>[2x]MRQIAIYGKGGIGKSTTTQNLTAALSTMGNNILLVGCDPKADSTRMLLGGLNQKTVLDTLRSEGDEGIDLDTVLQPGFGGIKCVESGGPEPGVGCAGRGIITSIGLLENLGAYTDDLDYVFYDVLGDVVCGGFAMPIREGKAKEIYIVASGELMAIYAANNICKGLAKFAKGGARLGGIICNSRKVDGERELLEAFAKKLGSHLIHFVPRDNIVQRAEINRKTVIDFDRESDQAKEYLTLADNVQNNNKLVVPTPLPMEELEAMMVEFGIVEL

A homodimer carrying a subunit-bridging [Fe4S4] cluster at the protein surface, the iron (Fe) protein of nitrogenase is best known for its function as an obligate electron donor for its catalytic partner during substrate turnover. Perhaps more interestingly, the Fe protein from a methanogenic microorganism, Methanosarcina acetivorans (designated MaNifH), was capable of reducing CO2 past CO into hydrocarbons under ambient conditions in the presence of EuII-DTPA, further illustrating the unique reactivity of the [Fe4S4] cluster toward CO2 (16, 17). Despite its archaeal origin, MaNifH shares a sequence identity of 59% and a sequence homology of 72% with AvNifH. Like AvNifH, MaNifH is a homodimer of ∼60 kDa, and it contains an [Fe4S4] cluster that can adopt three oxidation states upon redox treatments: (i) the oxidized state ([Fe4S4]2+), which is generated upon treatment by indigodisulfonate; (ii) the reduced state ([Fe4S4]1+), which is generated upon treatment by dithionite (DT); and (iii) the “superreduced,” all-ferrous state ([Fe4S4]0), which is generated upon treatment by EuII-DTPA.

Here, we report a 2.4-Å crystal structure of MaNifH that was generated in the presence of dithionite and an alternative CO2 source, bicarbonate. Consistent with the presence of its [Fe4S4] cluster in the +1 oxidation state, MaNifH crystallized in the presence of dithionite had a characteristic brown color. A closer examination of the region surrounding the active site of MaNifH reveals the ligation of the [Fe4S4] cluster by four Cys residues: two from subunit A (Cys95A, Cys130A) and two from subunit B (Cys95B, Cys130B). Interestingly, the electron density omit map (Fo − Fc) of the active site of MaNifH (Fig. 1C, green mesh) indicates the presence of additional electron density that lies immediately next to the crystallographic symmetry axis, seemingly held by two pairs of conserved Arg residues (R98A and R98B)—one from each of the two adjacent MaNifH subunit dimers. Similarly, CO2 could be modeled with reasonable R factor values at the crystallographic symmetry axis; only in this case, two molecules of CO2—each at 100% occupancy—could be assigned to the asymmetric unit and its symmetry mate, respectively. In this scenario, the CO2 moiety has its C atom placed at a distance of ∼4 Å from the nearest Fe atom (Fe-3) of the [Fe4S4] cluster, with the NH2+ groups of R98A and R98B assuming the “distal” and “proximal” positions, respectively, to Fe-3. This observation suggests a possible role of the conserved Arg pair in capturing CO2 via hydrogen bonding and/or electrostatic interactions, as well as a potentially asymmetric functionality of the two Arg residues in this process.> MGSLTEDGLSYKEKFVVRSYEVGSNKTATVETIANLLQEVGCNHAQSVGFSTDGFATTTTMRKLHLIWVTARMHIEIYKYPAWGDVVEIETWCQSEGRIGTRRDWILKDSVTGEVTGRATSKWVMMNQDTRRLQKVSDDVRDEYLVFCPQEPRLAFPEENNRSLKKIPKLEDPAQYSMIGLKPRRADLDMNQHVNNVTYIGWVLESIPQEIVDTHELQVITLDYRRECQQDDVVDSLTTTTSEIGGTNGSATSG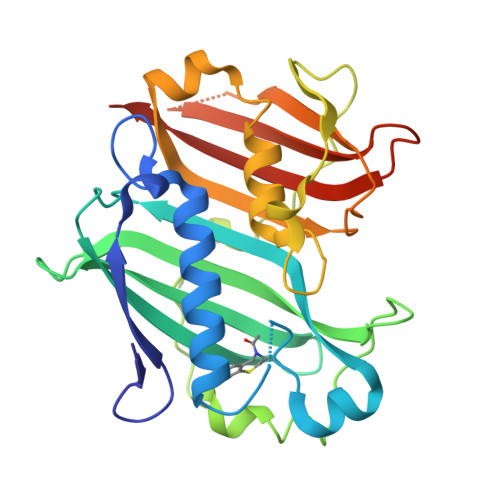TQGHNDSQFLHLLRLSGDGQEINRGTTLWRKKPSSHHHHHH> GGGCGCUGGU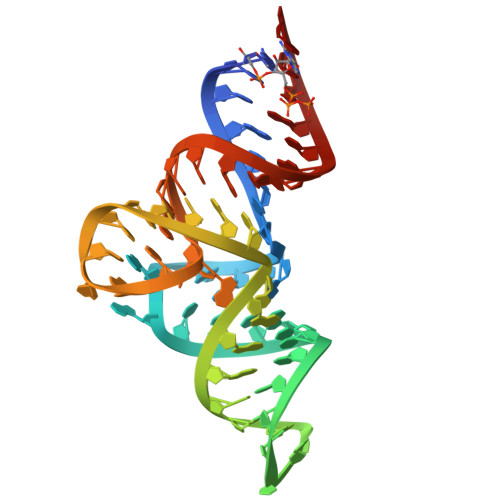GGUGGCACGUCCAGCACGGCUGGGCCGGGGUUCGAGUCCCCGCAGUGUUC>[4x]MVVKFMDVYQRSYCHPIETLVDIFQEYPDEIEYIFKPSCVPLMRAGGCCNDEGLE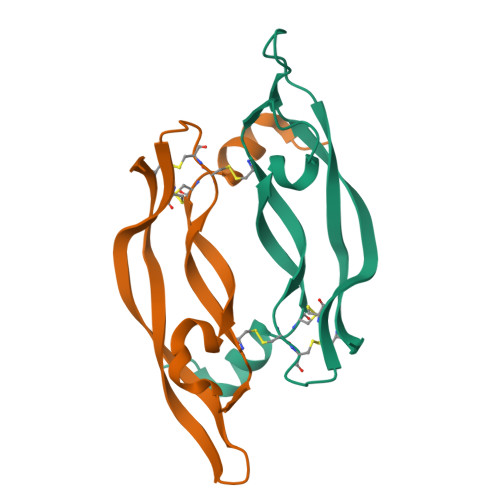CVPTEESNITMQIMRIKPHQGQHIGEMSFLQHNKAECRPKK> SSSGLVPRGSAMGKPQPIAAANWKCNGGGQSLSELIDLFNSTSINHDVQCVVAPSWYMGAQAMTKERLSHPKFVIAAQNAGNADALASLK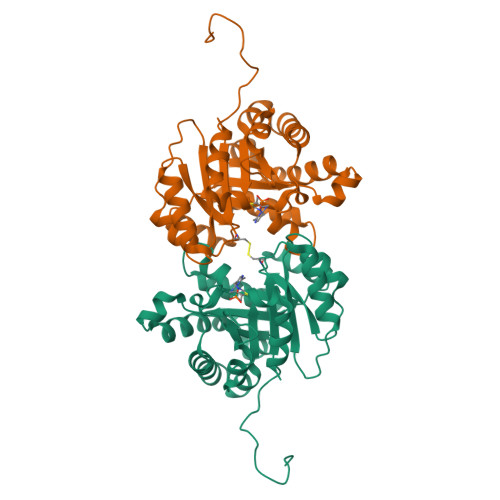DFGISWIVLGHSERRAYYGETNEIVADKVAAAVASGFMVIACIGETLQERSSGRTAVVVLTQITAIAKKLKKADWAKVVIAYEPVWAIGTGKVATPQQAQEAHALIRSWVSSKVGADVAGELRILYGGSVNGKNARTLYQQRDVNGFLVGGASLKPEFVDIIKATQ Ethambutol | C10 H24 N2 O2 | 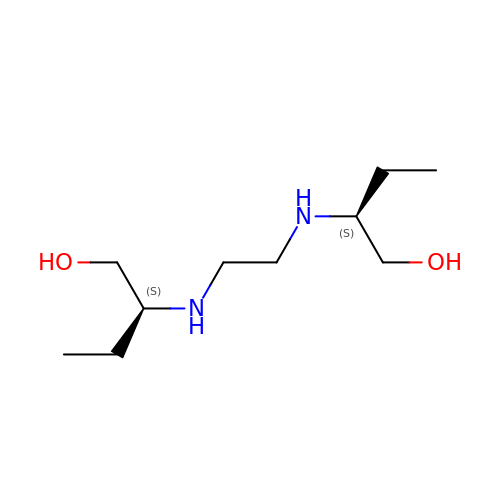AEUTYOVWOVBAKS-UWVGGRQHSA-N> MPSGNEEINHL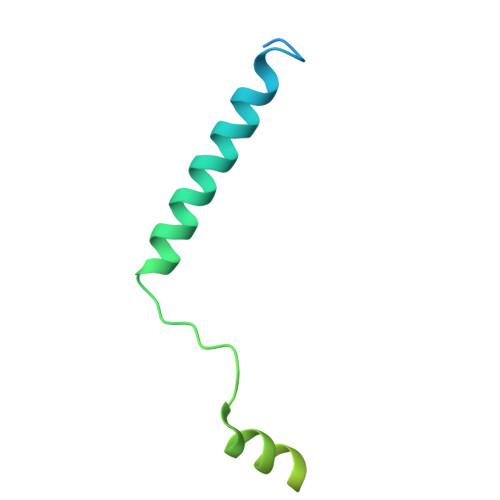SALDQFVAPGLRLWMLIALVGGVLLIMIVIVCCFMRIRIPRTKRQIDLIAAKRKLRKSTKNSAEANAHNDERAQAIVMNSMPSGGGGGAPSTSSSRHTGSRIQSQV>[2x]MRSRRVDVMDVMNRLILAMDLMNRDDALRVTGEVREYID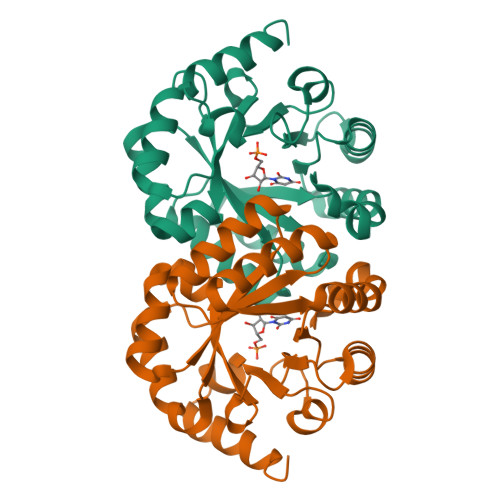TVKIGYPLVLSEGMDIIAEFRKRFGCRIIADFKVADIPETNEKICRATFKAGADAIIVHGFPGADSVRACLNVAEEMGREVFLLTEMSHPGAEMFIQGAADEIARMGVDLGVKNYVGPSTRPERLSRLREIIGQDSFLISPGVGAQGGDPGETLRFADAFIVGRSIYLADNPAAAAAGIIESIKDLLNP2-{[3-hydroxy-5-(octyloxy)benzyl]sulfanyl}benzoic acid | C22 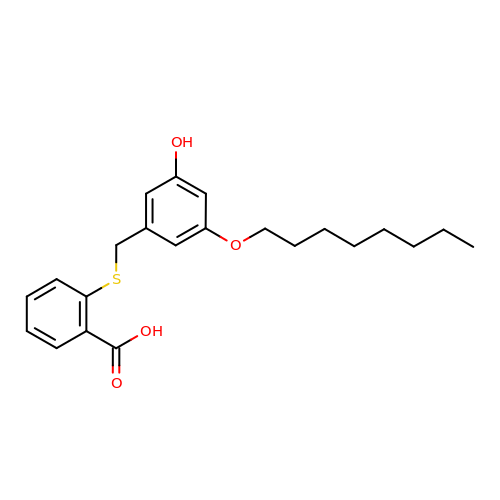H28 O4 S | VWFBKLSSSBBNHA-UHFFFAOYSA-N> MSSCINPSTLATSVNGFKCLPLATNRAAIRIMAKNKPVQCLVSTKYDNLTVDRRSANYQPSIWDHDFLQSLNSNYTDETYKRRAEELK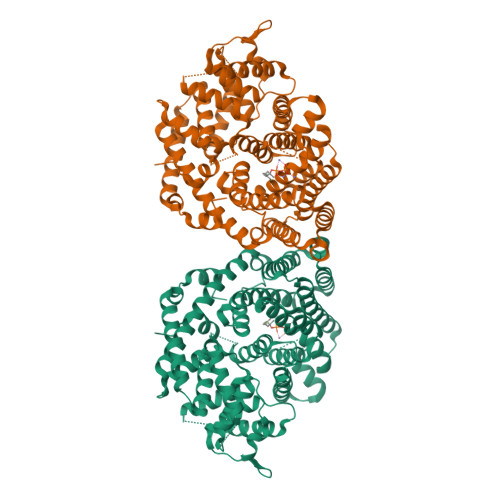GKVKTAIKDVTEPLDQLELIDNLQRLGLAYHFEPEIRNILRNIHNHNKDYNWRKENLYATSLEFRLLRQHGYPVSQEVFSGFKDDKVGFICDDFKGILSLHEASYYSLEGESIMEEAWQFTSKHLKEMMITSNSKEEDVFVAEQAKRALELPLHWKAPMLEARWFIHVYEKREDKNHLLLELAKLEFNTLQAIYQEELKDISGWWKDTGLGEKLSFARNRLVASFLWSMGIAFEPQFAYCRRVLTISIALITVIDDIYDVYGTLDELEIFTDAVARWDINYALKHLPGYMKMCFLALYNFVNEFAYYVLKQQDFDMLLSIKHAWLGLIQAYLVEAKWYHSKYTPKLEEYLENGLVSITGPLIITISYLSGTNPIIKKELEFLESNPDIVHWSSKIFRLQDDLGTSSDEIQRGDVPKSIQCYMHETGASEEVAREHIKDMMRQMWKKVNAYTADKDSPLTRTTAEFLLNLVRMSHFMYLHGDGHGVQNQETIDVGFTLLFQPIPLEDKDMAFTASPGTKG> GSHMKTLKPKEIKFNSWEELLKWEPGAREDDAINRGSVVLASRRTGHLVNEKASKEAKVQALSNTNSKAKDHASVGGEEFKAYAFDYWQYLDSMVFWEGLVPTPDVIDAGHRNGVPVYGTLFFNWS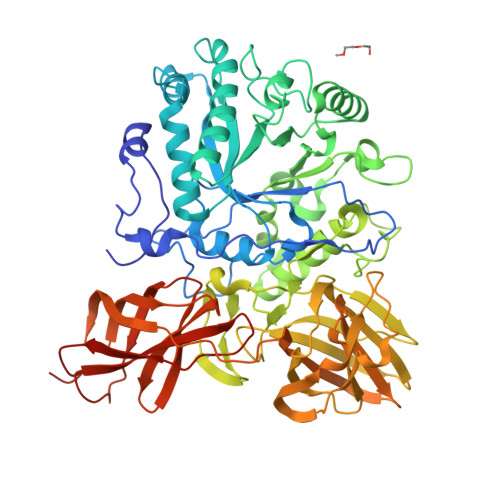NSIADQERFAEALKQDADGSFPIARKLVDMAKYYGYDGYFINQETTGDLVKPLGEKMRQFMLYSKEYAAKVNHPIKYSWYDAMTYNYGRYHQDGLGEYNYQFMQPEGDKVPADNFFANFNWDKAKNDYTIATANWIGRNPYDVFAGLELQQGGSYKTKVKWNDILDENGKLRLSLGLFAPDTITSLGKTGEDYHKNEDIFFTGYQGDPTGQKPGDKDWYGIANLVADRTPAVGNTFTTSFNTGHGKKWFVDGKVSKDSEWNYRSVSGVLPTWRWWQTSTGEKLRAEYDFTDAYNGGNSLKFSGDVAGKTDQDVRLYSTKLEVTEKTKLRVAHKGGKGSKVYMAFSTTPDYKFDDADAWKELTLSDNWTNEEFDLSSLAGKTIYAVKLFFEHEGAVKDYQFNLGQLTISDNHQEPQSPTSFSVVKQSLKNAQEAEAVVQFKGNKDADFYEVYEKDGDSWKLLTGSSSTTIYLPKVSRSASAQGTTQELKVVAVGKNGVRSEAATTTFDWGMTVKDTSLPKPLAENIVP> EPWAAAVPPEWV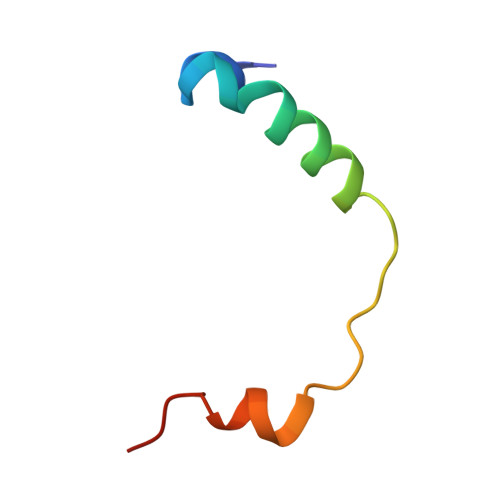PIIQQDIQSQRKVKPQPPLSDAYLSGMPAKR>[4x]MHHHHHHEEFRPEMLQGKKVIVTGASKGIGREMAYHLAKMGAHVVVTARSKET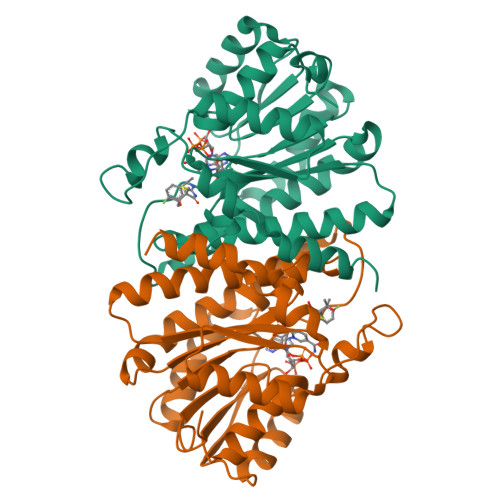LQKVVSHCLELGAASAHYIAGTMEDMTFAEQFVAQAGKLMGGLDMLILNHITNTSLNLFHDDIHHVRKSMEVNFLSYVVLTVAALPMLKQSNGSIVVVSSLAGKVAYPMVAAYSASKFALDGFFSSIRKEYSVSRVNVSITLCVLGLIDTETAMKAVSGIVHMQAAPKEECALEIIKGGALRQEEVYYDSSLWTTLLIRNPSRKILEFLYSTSYNMDRFINK>MKKIFMMVHELDVNKGGMTSSMFNRSKEFYDADIPADIVTFDYKGNYDEIIKALKKQGKMDRRTKMYNVFEYFKQISNNKHFKSNKLLYKHISERLKNTIEIEESKGISRYFDITTGTYIAYIRKSKSEKVIDFFKDNKRIERFSFIDNKVHMKETFNVDNKVCYQVFYDEKGYPYISRNINANNGAVGKTYVLVNKKEFKNNLALCVYYLEKLIKDSKDSIMICDGPGSFPKMFNTNHKNAQKYGVIHVNHHENFDDTGAFKKSEKYIIENANKINGVIVLTEAQRLDILNQFDVENIFTISNFVKIHNAPKHFQTEKIVGHISRMVPTKRIDLLIEVAELVVKKDNAVKFHIYGEGSVKDKIAKMIEDKNLERNVFLKGYTTTPQKCLEDFKLVVSTSQYEGQGLSMIEAMISKRPVVAFDIKYGPSD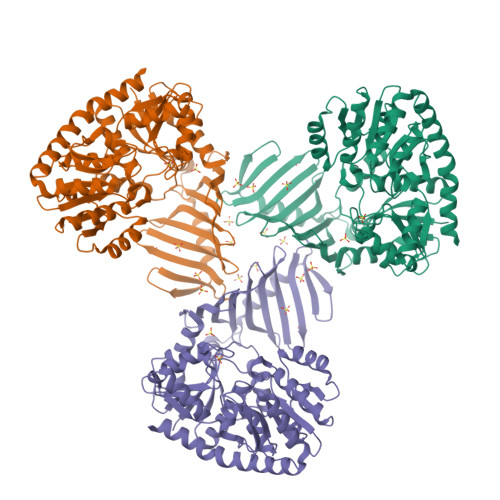FIEDNKNGYLIENHNINDMADKILQLVNNDVLAAEFGSKARENIIEKYSTESILEKWLNLFNS[2x]>MGGSGSRLSKELLAEYQDLTFLTKQEILLAHRRFCELLPQEQRSVESSLRAQVPFEQILSLPELKANPFKERICRVFSTSPAKDSLSFEDFLDLLSVFSDTATPDIKSHYAFRIFDFDDDGTLNREDLSRLVNCLTGEGEDTRLS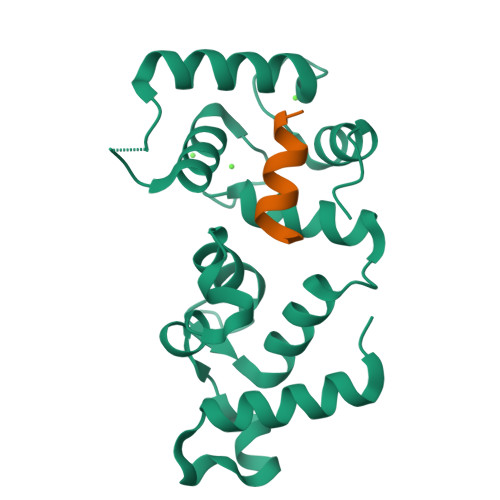ASEMKQLIDNILEESDIDRDGTINLSEFQHVISRSPDFASSFKIVL[2x];>[2x]SFWYGAMKALYG> SMGESRVILAFGDALFAGYGLDKGESYPAKLETALRSHGINARIINAGVSGDTTAAGLQRIKFVLDSQPDKPELAIVELGGNDLLRGLSPAEARQNLSGILEELQRRKI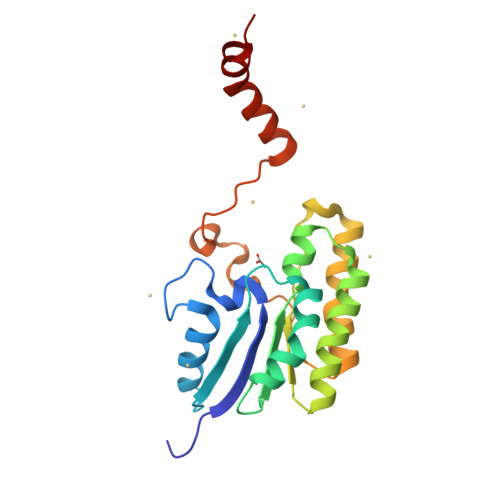PILLMGMRAPPNLGAKYQREFDGIYPYLAEKYDAKLVPFFLEAVADRPDLIQKDHVHPTARGVEELVSATSNAVAKALPAKK>MEHHHHHHATNLRGVMAALLTPFDQQQAL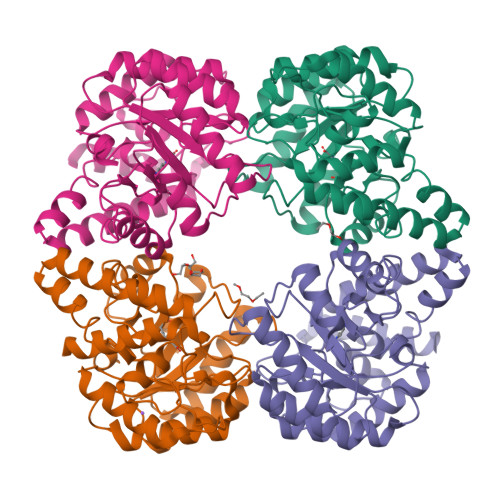DKASLRRLVQFNIQQGIDGLYVGGSTGEAFVQSLSEREQVLEIVAEEAKGKIKLIAHVGCVSTAESQQLAASAKRYGFDAVSAVTPFYYPFSFEEHCDHYRAIIDSADGLPMVVYNIPALSGVKLTLDQINTLVTLPGVGALKQTSGDLYQMEQIRREHPDLVLYNGYDEIFASGLLAGADGGIGSTYNIMGWRYQGIVKALKEGDIQTAQKLQTECNKVIDLLIKTGVFRGLKTVLHYMDVVSVPLCRKPFGPVDEKYLPELKALAQQLMQER[4x]> GSHMMKRLVYISKISGHLSLEEIQRIGKVSIKNNQRDNITGVLLYLQGLFFQILEGENEKVDKLYKKILVDDRHTNILCLKTEYDITDRMFPNWAMKTINLNENSELMIQPIKSLLQTITQSHRVLEKFMPARVIYLINQGINPLTVEPQLVEKIIFFSDILAFSTLTEKLPVNEVVILVNRYFSICTRIISAYGGEVTK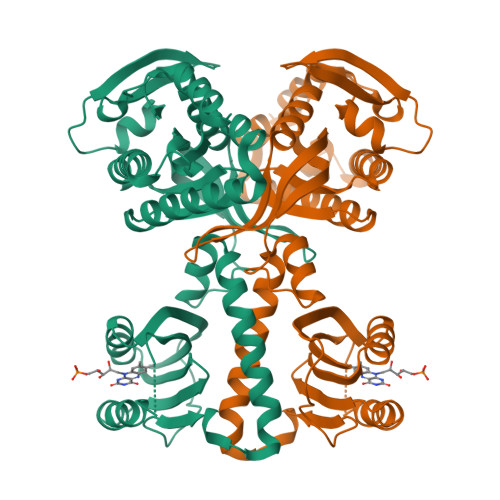FIGDCVMASFTKEQGDAAIRTSLDIISELKQLRHHVEATNPLHLLYTGIGLSYGHVIEGAMGSSLKMDHTLLGDAVNVAARLEALTRQLPYALAFTAGVKKCCQAQWTFINLGAHQVKGKQEAIEVYTVNEAQKYYDTLQITQLIRQTLENDK>[2x]MGDKPIWEQIGSSFINHYYQLFDNDRTQLGAIYIDASCLTWEGQQFQGKAAIVEKLSSLPFQKIQHSITAQDHQPTPDSCIISMVVGQLKADEDPIMGFHQMFLLKNINDAWVCTND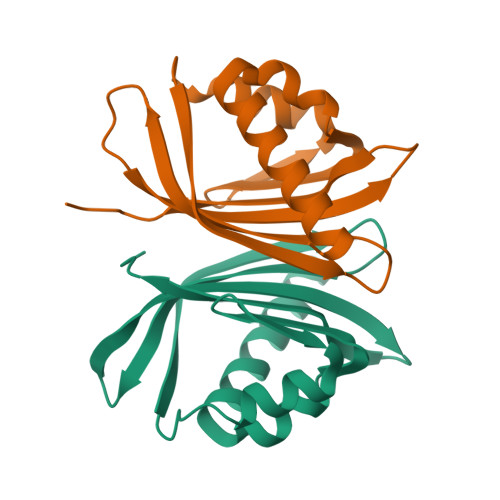EFRLALHNFG> GH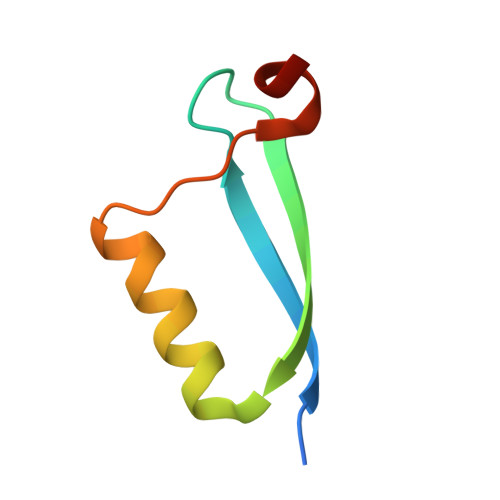MAEPQRHTMLCMCCKCEARIELVVESSADDLRAFQQLFLNTLSFVCPWCASQQ> ESPLPKPVLDTNGKELNPDSSYR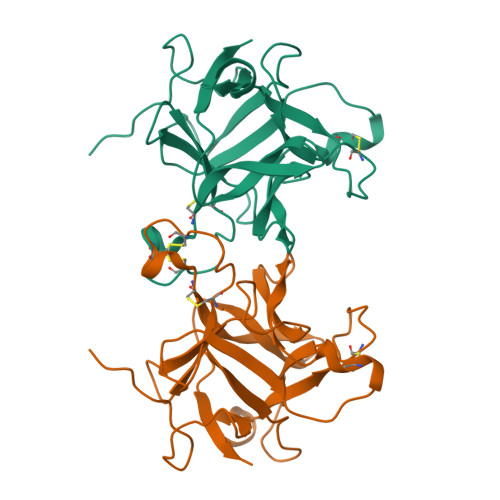IISIGRGALGGDVYLGKSPNSDAPCPDGVFRYNSDVGPSGTPVRFIPLSTNIFEDQLLNIQFNIPTVKLCVSYTIWKVGNLNAYFRTMLLETGGTIGQADNSYFKIVKSSKIGYNLLSCPFTSIICLRCPEDQFCAKVGVVIQNGKRRLALVNKNPLDVLFQEV>CSTVSPGVLAGIVVGDLVLTVLIALAVYFLGRL[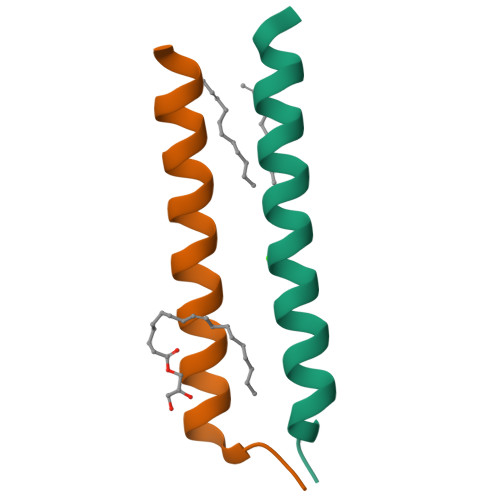4x]> MAVTNEEIKTASKIVRRVSNVEAFDKSGSVFKGYQIWTDISPTIENDPNIMFVKCVVQQGSKKEKLTVVQI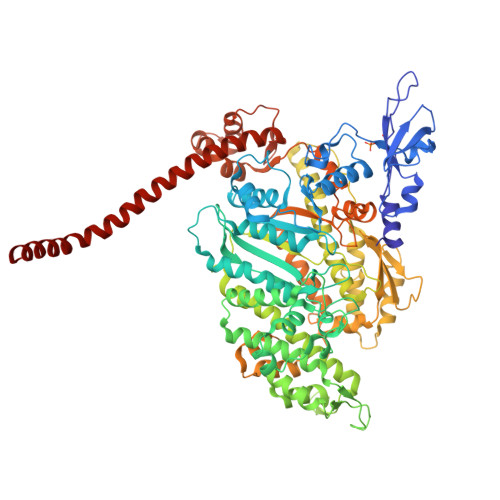DPPGTGTPYDIDPTHAWNCNSQVDPMSFGDIGLLNHTNIPCVLDFLKHRYLKNQIYTTAVPLIVAINPYKDLGNTTNEWIRRYRDTADHTKLPPHVFTCAREALSNLHGVNKSQTIIVSGESGAGKTEATKQIMRYFASSKSGNMDLRIQTAIMAANPVLEAFGNAKTIRNNNSSRFGRFMQLVISHEGGIRYGSVVAFLLEKSRIITQDDNERSYHIFYQFLKGANSTMKSKFGLKGVTEYKLLNPNSTEVSGVDDVKDFEEVIESLKNMELSESDIEVIFSIVAGILTLGNVRLIEKQEAGLSDAAAIMDEDMGVFNKACELMYLDPELIKREILIKVTVAGGTKIEGRWNKNDAEVLKSSLCKAMYEKLFLWIIRHLNSRIEPEGGFKTFMGMLDIFGFEVFKNNSLEQLFINITNEMLQKNFVDIVFERESKLYKDEGISTAELKYTSNKEVINVLCEKGKSVLSYLEDQCLAPGGTDEKFVSSCATNLKENNKFTPAKVASNKNFIIQHTIGPIQYCAESFLLKNKDVLRGDLVEVIKDSPNPIVQQLFEGQVIEKGKIAKGSLIGSQFLNQLTSLMNLINSTEPHFIRCIKPNENKKPLEWCEPKILIQLHALSILEALVLRQLGYSYRRTFEEFLYQYKFVDIAAAEDSSVENQNKCVNILKLSGLSESMYKIGKSMVFLKQEGAKILTKIQREKLVEWENCVSVIEAAILKHKYKQKVNKNIPSLLRVQAHIRKKMVAQ>[2x]MGAHASVIKPEMKIKLRMEGAVNGHKFVIEGEGIGKPYEGTQTLDLTVEEGAPLPFSYDILTPAFEYGNRAFTKYPEDIPDYFKQAFPEGYSWERSMTYEDQGICIATSDITMEGDCFFYEIRFDGTNFPPNGPVMQKKTLKWEPSTEKMYVEDGVLKGDVEMALLLEGGGHYRCDFKTTYKAKKDVRLPDAHEVDHRIEILSHDKDYNKVRLYEHAEAR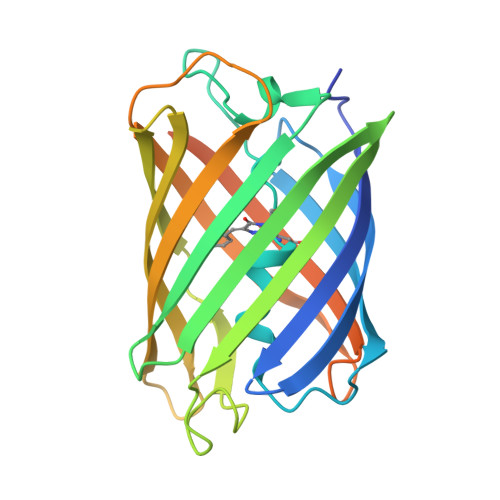YSGGGSGGGASGKPIPNPLLGLDSTHHHHHH> MSDMNNPSDENTGALDDLWADALNEQKATTTKSAADAVFQQLGGGDVSGAMQDIDLIMDIPVKLTVELGRTRMTIKELLRLTQGSVVALDGLAGEPLDIL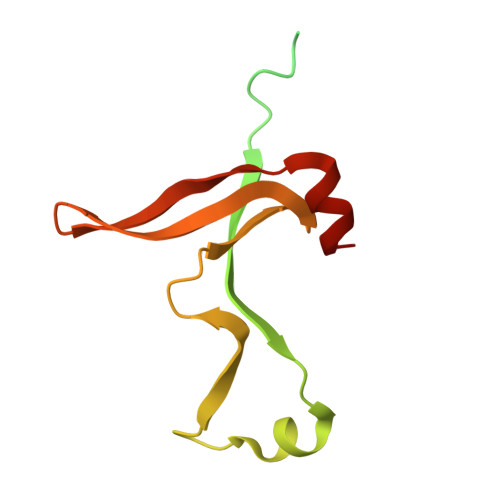INGYLIAQGEVVVVADKYGVRITDIITPSERMRRLSR> EDSFLQR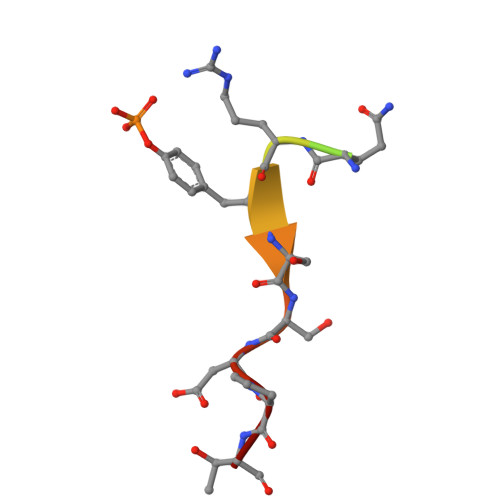YSSDPT>GAMVSQPIKLLVGLANPGPEYAKTRHNAGAWVVEELARIHNVTLKNEPKFFGLTGRLLINSQELRVLIPTTFANLSGKAIAALANFYQIKPEEIMVAHDELDLPPGVAKFKQGGGHGGHNGLKDTISKLGNNKEFYRLRLGIGHPGHKDKVAGYVLGKAPAKEQECLDAAVDESVRC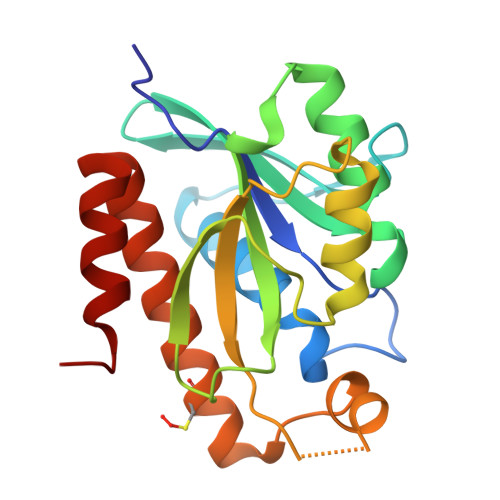LEILMKDGLTKAQNRLHTFKAE[2x]> SHMASSWDEMSCAEKLLKVLSFGLWNPTYSRSERQSFQELLTVLEPVYPLPNELGRVSARFSDGSSLRISVTNSESIEAEIRTPDNEKITVLLESNEQNRLLQSLPIDRHMPYIQVHRALSEMDLTDTTSMRNLLGFTSKLSTTLIPHNAQTDPLSGPTPFSSIFMDTCRGLGNAKLSLNGVDIPANAQMLLRDALGLKDTHSSPSRNVIDHGISRHDAEQIARESSGSDN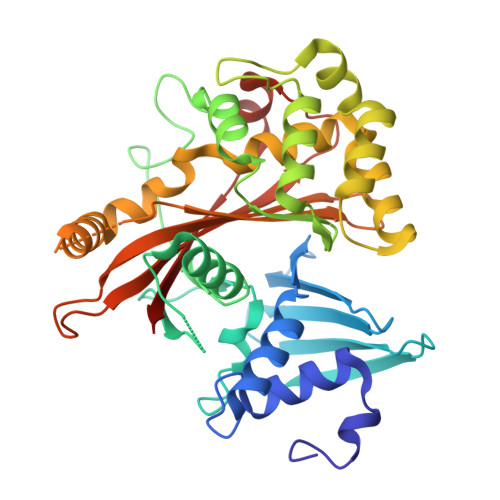QKAEVVEFLCHPEAATAICSAFYQSFNVPALTLTHERISKASEYNAERSLDTPNACINISISQSSDGNIYVTSHTGVLIMAPEDRPNEMGMLTNRTSYEVPQGVKCTIDEMVRALQPRYAASETYLQNT>MSAVALPRVSGGHDEHGHLEEFRTDPIGLMQRVRDELGDVGTFQLAGKQVVLLSGSHANEFFFRAGDDDLDQAKAYPFMTPIFGEGVVFDASPERRKEMLHNAALRGEQMKGHAATIEDQVRRMIADWGEAGEIDLLDFFAELTIYTSSACLIGKKFRDQLDGRFAKLYHELERGTDPLAYVDPYLPIESFRRRDEARNGLVALVADIMNGRIANPPTDKSDRDMLDVLIAVKAETGTPRFSADEITGMFISMMFAGHHTSSGTASWTLIELMRHRDAYAAVIDELDELYGDGRSVSFHALRQIPQLENVLKETLRLHPPLIILMRVAKGEFEVQGHRIHEGDLVAASP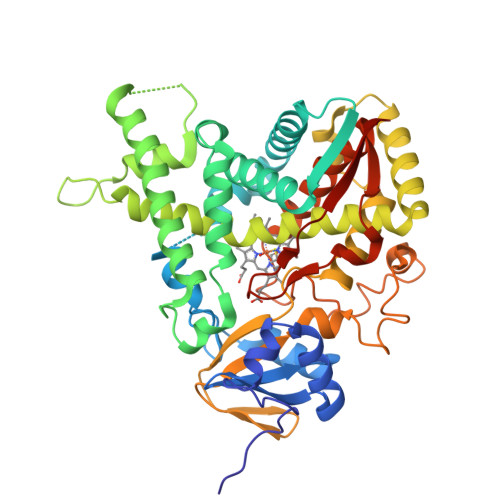AISNRIPEDFPDPHDFVPARYEQPRQEDLLNRWTWIPFGAGRHRCVGAAFAIMQIKAIFSVLLREYEFEMAQPPESYRNDHSKMVVQLAQPAAVRYRRRTGVHHHH[2x]>[3x]MVELDKYLPVNREEAFRNGVNKNFAKIEQGFSQRDAVMNSHQTTQKNAHDTEQILHYLSDKEKD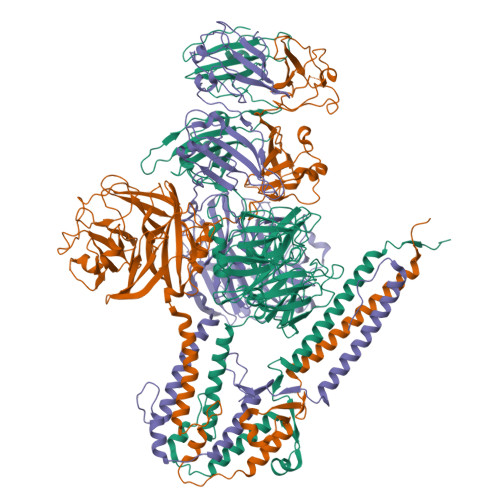VYYHSALDLKHYLLLECSRISNLVLGATTDQSVELKESRVDLEGKAHITLYGRLLADFTRLKNALDKLIELEESFDIPKIEPQFWTELGGIRNVVQQYFWINKLNGRVYQTQSDSQAQEGFYINELTPSGHFLGTMHIPKGGHGTSLGVEYVNGQMFMWTNVDKRLVKFTFKADTKLDATLLRDYMPSSVAPVFFAPVSDWKGEKMAFRRSDGIIELRDVNDLNKNIDKVYAQVTIPLEERENDYRPMQGVAISDKNCYWMSGWGTDENIGKVFVYDWHGKLLDTITLDNLTQVTGVGGEEYASDNHSEPEGLFFTEDKGKKVLFVGFSTGGTRKRHHKIYGFSQRGGLERYSSIVRNGAQNYPLTRGDGKAHSTPDGLTKLSDLTKVGSYYAQGSDVALLTDLPVEFKGVPLWIDNLPAEQHNDVRQVITRRSTEKSMLKFERMINIGKAEQAFSVGSWTVYQSQTTRGEFIDASIYQNKLSNITSPMKMYMTAEQANLFTDHPVKNGNAGWFYENSGYGVTGEFRQTITINSSLRYEVYSRMVFADRVSEWFVIAGNQVK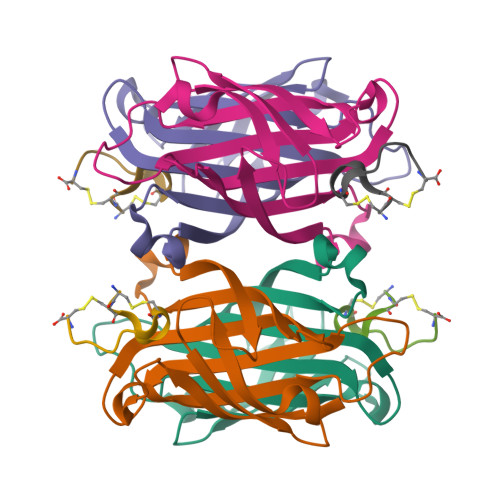>[4x]GAAEAGITGTWYNQLGSTFIVTAGADGALTGTYESAVGNAESRYVLTGRYDSAPATDGSGTALGWTVAWKNNYRNAHSATTWSGQYVGGAEARINTQWLLTSGTTEANAWKSTLVGHDTFTKVKPSAAS;>[4x]CCHPQCGAAYSC> MRFKKHVVQHEETMQAIAQRYYGDVSYWIDLVEHNNLKYPYLVETDEEKMKDPERLASTGDTLIIPIESDLTDVSAKEINSRDKDVLVELALGRDLNITADEKYFNEHGTSDNILAFSTNGNGDLDTVKGIDNMKQQLQARLLTPRGSLMLHPNYGSDLHNLFGLNIPEQATLIEMEVLRTLTSDNRVKSANLIDWKIQGNVYSGQFSVEIKSVEESINFVLGQDEEGIFALFE;>[2x]MKTRKLTNILSKLIDKTMAGTSKITDFTPGSASRSLLEAVSLEIEQFYILTKENIDWGIQEGIIEAFDFQKRQSKRAYGDVTIQFYQPLDMRMYIPAGTTFTSTRQEYPQQFETLVDYYAEPDSTEIVVEVYCKETGVAGNVPEGTINTIASGSSLIRSVNNEYSFNTGTKEESQEDFKRRFHSFVESRGRATNKSVRYGALQIPDVEGVYVYEETGHITVFAHDRNGNLSDTLKEDIIDALQDYRPSGIMLDVTGVEKEEVNVSATVTISNKSRIGDTLQKHIESVIRSYLNNLKTSDDLIITDLIQAIMNIDDVLIYDVSFDNLDENIIVPPQGIIRAGEIKVELK;> MANFLKNLHPLLRRDRNKKDNQDPNFALIDALNEEMNQVEKDAIESKLQSSLKTSTSEYLDKFGDWFGVYRKTDEKDDVYRARIIKYLLLKRGTNNAIIDAIKDYLGRDDIDVSVYEPFTNIFYTNKSHLNGEDHLMGYYYRFAVINVSIGDYFPVEIIDVINEFKPAGVTLYVTYDGASTIRGGAIIKWLDGLPKIETYQEFDRFTGYDDTFYGHINMNQSKDTDNSSSDIFKTNHSLINSLDVLTGSSSVGRQYINYGYVTSYVYNPGMTSSVNQISASTEGRGQEVPTDYYMYTSTKNNNTVELSMQTTSGVSYLYNNFNFRDYMSKYRPQVDLQSDEARRI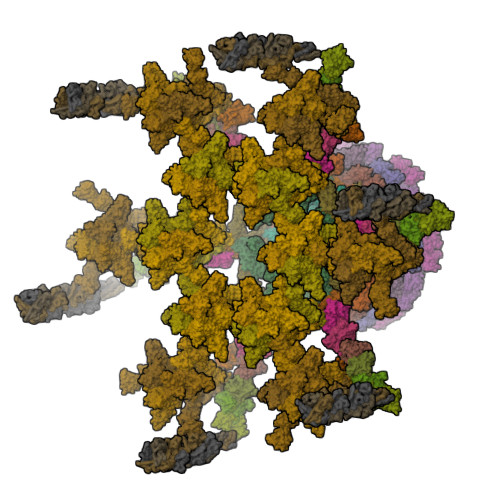VSDYIKELSIDYYLSAVIPPDESIEIKLQVYDFSINRWLTVSINNLSFYEKNIGSNIGYIKDYLNSELNMFTRLEINAGKRDSVDIKVNYLDLMFYYYERGIYTIKPYKALIENYLDISRETYVEAFKIASLSNGDIITKTGFQPIGYLKLVGNYENTIPSTINIVAKDTDNNPIESNELDVYNTVENRNLLQSYKGVNTIAREITSTKEFTVSGWAKEIYSTNYLSKVLKPGKVYTLSFDMEITGNDPTLKSYSDNHGIYLYSNTKGIVVNGVKSMERTIGNKVSVTQTFTAPTITDHRLLIYTGRYTSDGKASTPPVFFNTVKITELKLTEGSSKLEYSPAPEDKPNVIEKGIKFNNILTNIQTLSINSDTILKNVTLYYSYYGDSWVELKTLGNISTGETTETNNLIDLYGLQTVDYSNINPMSKVSLRSIWNVKLGELNNQEGSLSNMPNDYFNAVWQDIDKLSDIELGSMRMVKDTEGGVFDGATGEIIKATLFNVGAYTDLDMLAYTLTNYTEPLTLGSSRLISELKEELLTSESFNVDNRIKVIDSIYEELPNTSIIKNGFVEREVTGSKYLDYGLYEPIEDGTRYKLIVEGEFKDNIEFISLYNSNPNFNETFIYPSEIINGVAEKEFIAKPSTEDKPRLNTDVRIYIRPYDSTISKVRRVELRKV;>MAVEPFPRRPITRPHASIEVDTSGIGGSAGSSEKVFCLIGQAEGGEPNTVYELRNYSQAKRLFRSGELLDAIELAWGSNPNYTAGRILAMRIEDAKPASAEIGGLKITSKIYGNVANNIQVGLEKNTLSDSLRLRVIFQDDRFNEVYDNIGNIFTIKYKGEEANATFSVEHDEETQKASRLVLKVGDQEVKSYDLTGGAYDYTNAIITDINQLPDFEAKLSPFGDKNLESSKLDKIENANIKDKAVYVKAVFGDLEKQTAYNGIVSFEQLNAEGEVPSNVEVEAGEESATVTATSPIKTIEPFELTKLKGGTNGEPPATWADKLDKFAHEGGYYIVPLSSKQSVHAEVASFVKERSDAGEPMRAIVGGGFNESKEQLFGRQASLSNPRVSLVANSGTFVMDDGRKNHVPAYMVAVALGGLASGLEIGESITFKPLRVSSLDQIYESIDLDELNENGIISIEFVRNRTNTFFRIVDDVTTFNDKSDPVKAEMAVGEANDFLVSELKVQLEDQFIGTRTINTSASIIKDFIQSYLGRKKRDNEIQDFPAEDVQVIVEGNEARISMTVYPIRSFKKISVSLVYKQQTLQA[6x];>[6x]MAIATYNSHVELAKYLVSKADSVYLTIGKSTPWSNETNPPQPDENATVLQEVIGYKKATKVTLVRPSKSPEDDNKNLISYGNKSWVEVTPENAKAEGAKWVYLESSIVGDELPLGTYRQVGFVMDLVAKSGISKFNLVPSEVESTGTLLFFDNKQFQNRSEQTTAKERFIVEVDPNSSSVDKLAAALEHHHHHH;>[6x]MAINFKGSPYLDRFDPSKDRTKVLFNPDRPLQQAELNEMQSIDQYYLKNLGDAIFKDGDKQSGLGFTLSEDNVLTVNPGYVYINGKIRYYDNDDSVKITGVGKETIGIKLTERIVTPDEDASLLDQTSGVPSYFSKGADRLEEKMSLTVNDPTSATIYTFMDGDLYIQSTNAEMDKINKVLAERTYDESGSYKVNGFELFSEGNAEDDDHVSVVVDAGKAYVKGFKVDKPVSTRISVPKSYDLGTAENESTIFNKSNNSISLANSPVKEIRRVTGQVLIEKERVTRGAQGDGQDFLSNNTAFEIVKVWTETSPGVTTKEYKQGEDFRLTDGQTIDWSPQGQEPSGGTSYYVSYKYNKRMEAGKDYEVTTQGEGLSKKWYINFTPSNGAKPIDQTVVLVDYTYYLARKDSVFINKYGDIAILPGEPNIMRLVTPPLNTDPENLQLGTVTVLPDSDEAVCISFAITRLSMEDLQKVKTRVDNLEYNQAVNALDDGAMEGQNPLTLRSVFSEGFISLDKADITHPDFGIVFSFEDAEATLAYTEAVNQPKIIPGDTTAHIWGRLISAPFTEERTIYQGQASETLNVNPYNIPNKQGVLKLTPSEDNWIDTENVTITEQKTKKVTMKRFWRHNESYYGETEHYLYSNLQLDAGQKWKGETYAYDREHGRTGTLLESGGQRTLEEMIEFIRIRDVSFEVKGLNPNDNNLYLLFDGVRCAITPATGYRKGSEDGTIMTDAKGTAKGKFTIPAGIRCGNREVTLKNANSTSATTYTAQGRKKTAQDIIIRTRVTVNLVDPLAQSFQYDENRTISSLGLYFASKGDKQSNVVIQIRGMGDQGYPNKTIYAETVMNADDIKVSNNASAETRVYFDDPMMAEGGKEYAIVIITENSDYTMWVGTRTKPKIDKPNEVISGNPYLQGVLFSSSNASTWTPHQNSDLKFGIYTSKFNETATIEFEPIKDVSADRIVLMSTYLTPERTGCTWEMKLILDDMASSTTFDQLKWEPIGNYQDLDVLGLARQVKLRATFESNRYISPLMSSSDLTFTTFLTELTGSYVGRAIDMTEAPYNTVRFSYEAFLPKGTKVVPKYSADDGKTWKTFTKSPTTTRANNEFTRYVIDEKVKSSGTNTKLQVRLDLSTENSFLRPRVRRLMVTTRDE;>MALNFTTITENNVIRDLTTQVNNIGEELTKERNIFDITDDLVYNFNKSQKIKLTDDKGLTKSYGNITALRDIKEPGYYYIGARTLATLLDRPDMESLDVVLHVVPLDTSSKVVQHLYTLSTNNNQIKMLYRFVSGNSSSEWQFIQGLPSNKNAVISGTNILDIASPGVYFVMGMTGGMPSGVSSGFLDLSVDANDNRLARLTDAETGKEYTSIKKPTGTYTAWKKEFEPKDMEKYLLSSIRDDGSASFPLLVYTSDSKTFQQAIIDHIDRTGQTTFTFYVQGGVSGSPMSNSCRGLFMSDTPNTSSLHGVYNAIGTDGRNVTGSVVGSNWTSPKTSPSHKELWTGAQSFLSTGTTKNLSDDISNYSYVEVYTTHKTTEKTKGNDNTGTICHKFYLDGSGTYVCSGTFVSGDRTDTKPPITEFYRVGVSFKGSTWTLVDSAVQNSKTQYVTRIIGINMP[3x]>MPRKKDQVTKNDDGNQTSDVQTQDFKTAVQPDTNTAQLIKTYSNPKQRGDKGEIIYDGGLSSKLADVVDKTTEPHNADGAVKDGRIAPVKLDLEKQKLDKLKLFETSPFDPLTIKNNQDVVDKLYATQSSSIQEVVPTKTFATELQFGVTSEDMAKIYGAVAAVSKNVNSSVTYEVKRGTHELIKVPTIPHNLVLIQSDNGKHALIKEDLGQWPVETGISLVNQAGVFAVQLANKLGIDKPFVLDAGSNYFTDTSFIDTRKYCTDGLSPREIQKALNRQRAYYDRPELTISENKTLLSQSIIYPDADGNDVSIIFSGAMSHAIFTYAQSQWNKNIIKLDDYIREITLTVPKQYRPRRFKEIEHTHGYVYRELNQGSLLPLVDANLKESSSYYFKKLMSSISNVPVDARTLQSATAALAADTGQAVNRAQHVSMLTNRLTTANAPTVRAITVLTCMFKQFRIGMTYALDPNIMDVAAATCMLLFRPAQSISDEQYRYCLQTMAVFLTNTTYDIVNNDTIDVLKMKLRNQGWPFVERYNAVEIDMSVEPLRSPGQVGRYYNPFNIDPLTKKHVEDRLEEFINQVQVGRFRNASGNAVGTTLAAFLRACRDKTSANWRGYSVLVSRYRSLIPNELFESLRNISGEYNINPQDEHSFFFALAQINADDEFIGAIDKESAEYLDEYATLARDISNSLTLVKAAFGPLERTSGSIINHANNLNKVINHVFADKPLISETMLKILTIDGTTGKDGYRNWLDKLVGHNYPVYVEPVVNIMNFISARFVADSSYFGYTNEIMIMPNHINVPVDDRFGFRDSPFCTSLPRTIMGNDVRRISYNVFSMMEDIDDVISEGFILYDAYFNFSYDIMTTDGVTRLKEDILIVTDTGNDIKPIHFYIYFENRNDKKLRYESKMNVSYRLYIKTPACLLPLSDYMRAQHDYVSPSSSRVYIKDPAVVYTRS[2x];>MANRATSAFLDNPHPVGVNYVDEGSRQFVAVAELLASKLIDSSRESDESNSDVPFVQAYSKFADDNPRHLR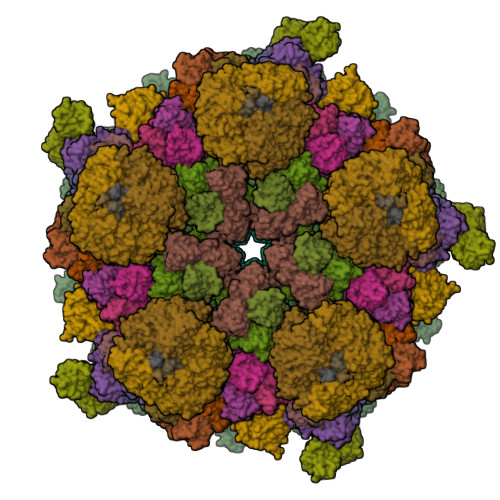VKTGGKMANALTNVIRSYYSINAPAIVPQVEIDRLASKATVSGDMYNSYAIFNSVPIVEVLSPARTTVSIVGSDRADVTMLNTGAGAANITFNFGQIAETVILKGSVPFQLARLNQPMPAARFTYKLRPLDGPFIVVLPVGNPLVISATAATRIQVPLAFNKALVESGFQTAMNDGLFDIQNVNYYSSFDEFIISQYHAQDGINRVSTCVILGLALQAYDQMRRALPVRRV[13x];>MDVLSKGSLKELLAHLEKTPLEEAISYRIGTVPYQNVLISRNEYYNQLYPDTTSLIDGVSREGQRNVNGLIMSIISYVVSGSGHYIPNIGFMLLRRSILDILTKHDTGLVTNNLNYGIIARNLTVSKMNCEQRKRMLICFKLLAYKDGNQNDYEIYLNQNIPLKQIAPNFIPGDMRTVIHNQDQLAIVGIPAYRLTQSTELSIRDDNAKSYKLGYVDWYNSNSFLRERSEFNLIRLKDRDTKYGKLNGW[2x];>MAWVTQAYSSGLSQNSIISLTGNDRTVADGTFNSMIMPRAVIANEREHFMKTRIDKIEHDLNRSAKQEMMDRQSLAEDYNALNLAVGQEIKLDIATQHQLNRLGSAMYKADHERETELTDLINRIRENEVTVNGILENQKAITAAERADLLLEVVASTAKSVSAAGRAAADGSGVVPVFGPSVANGIKVGIDIADSVAEAAIAVKESGIITQLNDVYHAFQSVHVAPNDVIKPAAVVAGTSTELIGNLQAIYSRLRSHSDIGFKKATVGDVIPNSYMIKPVNSTEYASWQLYVIHPVQGSLGLVVQLMGDALTYNVFAQYGNTSASEFGKTVLTGGATNTALEGTKVKFQTKVTAQQALALTMALKDAASMLSQGELIGYFEQYINLALEPDNLSLQDNMHKYHHLLTSQNSPIDWNYHDEEMHKWLDSRKTTNYDAMQKKDGTVIADIHIPKVFNDLRNTTLHCKLEGKQTIAGYTVYEYLIGPWAHYGDIDYSVVVDTLNEETKWYCEVIGIDGHLLIEKSVQHKPEKILELTVNDSGVTSFNGRNHDRLKLKVYVKDSLSVKVFRNWIGINAPRVKTKMFNDHIGVKYDYSHFDKNISPAHLTLTDLGWHTWDQYNAGNWTNIKP[3x];>MLSETELRALKKLSTTTSRVVGDSTLALPSNVKLSKGEVEKIAVTKKEMFDELAQCNLPTIELITREHTFNGDVIRFAAWLFLMNGQKLMIANNVAVRMGMQYATNLAGNNVKITYVTSNNVVKLGHIAAGVLANPYSNKGSGLFITYEYNLISNLIETGKVCVLFITSLSTTASSTNSFAYSTCSVPIENWDFNMIKLTAETSCASLTAMTNLVNSLVPGERTRPVGLYVDIPGVTVTTSASSGSLPLTTIPAVTPLIFSAYTKQVEEVGVINTLYALSYLP[3x]N-[3-(dimethylamino)propyl]-1-[(1r,3r)-3-(methylcarbamoyl)cyclobutyl]-2-(3,4,5-trimethoxyphenyl)-1H-1,3-benzimidazole-6-carboxamide 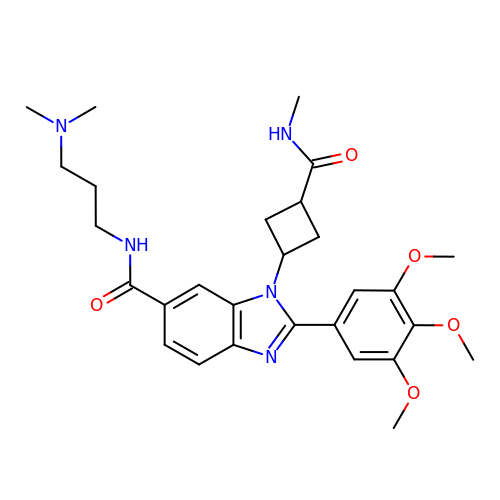| C28 H37 N5 O5 | COJOXDOWRKQNIY-MXVIHJGJSA-N> MK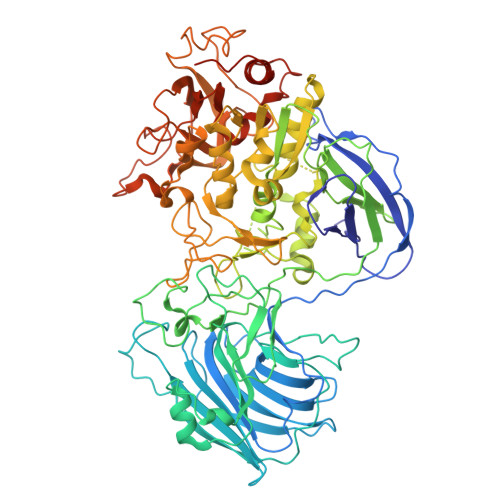DIAIRGYCDRPSVATGETIRFYVSANETRGTFDAELVRLIHGDSNPAGPGYKEEAIKSDLEGQYPARFQRTQFGSYVEVADPDAGLQPDGAFSVHLFLWSTTPSRGRQGIASRWNDERQSGWNLAIEDGRVVFTIGDGSGATSSVVSDRPLFQQIWYSITGVYDPEKKQLRLYQKSVVNRTNSRFGLVVPLDSDCAVSADATVKAADSETSLLIAGLGEAAAQDGRTWCIAHYNGKVDAPKIYGCALGQDDAEKLSRGEIVRPISRLAHWDFSAGIGLNGIPTDHVVDASGYGHHGRCMNQPSRGSTGWNWDGHEENFIHCPEQYGALWFHEDCLDDCRWEKDFEFTVPEGLKSDFYAVKIRYEDTEDYIPFFVLPPRGTATAPILVIASTLSYLAYANEQIMHKADIGQAVAGHTPVLNENDVELHKNLSYYGLSTADGHIDGRGVQYTSWRRPIMNLRPKHRQGFGSIWELPADLHLIDWLNHNGFEYDVATEHDLNDQGAELLRRYKVVLTGSHPEYQTWANADAWEDYLADGGRGMYLAANGMYWIVEVHPEKPWVMEVRKELGVTAWEAPPGEYHYSTNGRRGGRFRGRARATQKIWGTGMSSFGFDHSGYFVQMPDSQDERVAWIMEGIDPEERIGDGGLVGGGAGGYELDRYDLALGTPPNTLLLASSVEHSVVYTVIPDDKAFPHPGMNGGEHPFVRADITYFSTANGGGMFATSSISWLGSLSWNDYDNNVSKMTKNVLNQFIKDEPAPRVKLAAALEHHHHHH>[2x]RPRGPRAVFILPVTAQGEAVLIRQFRYPLRATITEIVAGGVEKGEDL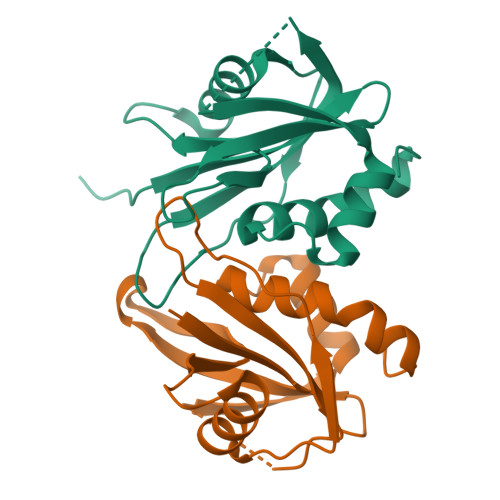GAAAARELLEEVGGAASEWVPLPGFYPQPSISGVVFYPLLALGVTLGAAQLEDTETIERVVLPLAEVYRMLEAGEIQDGPSSLTLWQARGELTRRGLL>MAHHHHHHMSKINKLEQIRNIGICAHIDAGKTTTTERILYYTGKSHKIGEVHEGGATMDWMEQEQERGITITSAATTCRWQDKVINIIDTPGHVDFTIEVERSLRVLDGAVAVFDGVAGVEPQSETVWRQADKYNVPRMCFVNKMDRMGADFYRCVEMIKDRLGARSLIIQLPIGIEENFKGIVNLIKMKAVIWKDESLGAEYFEEDIPADMQDKAAEYRARLLDMVVELDDTIMEQYLSGAEITEEQIKILIRKGTIEARFYPILCGSAFKNKGVQPLLDAIVDFLPSPIDIGIVKGIEVSTSEEKDFPISIVEPFSALAFKIMNDPFVGSLTFIRIYSGKITSGATVINTVKNKREKIGRMLLMHANNREDIKEASAGDIVALAGLKDTSTGDTLSDIDKQVVLERMEFPEPVIELAVEPKSTADQEKMGLALSRLAAEDPSFRVSTDHETGQTVIKGMGELHLEIIIDRMRREFKVEANIGAPQVAYRETITTACEIDYTHKKQSGGAGQFARVKIIFEPLKDVI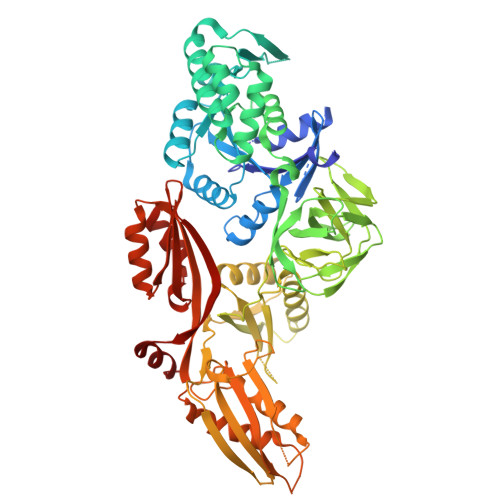DLKDEDKNKTFVFESKIVGGAVPKEYIPGVEKGLNNIRETGVIAGYPMIDFKATLVDGAFHDVDSSVLAFEIAAKGAFREGMQKGNPKLLEPIMKVEVITPDEYMGDIIGDLNSRRGQIQNMDPRGNAQVVTAHVPLAEMFGYVNTLRSLSQGRAQFSMIFSHYDQVPSQVADMIKAKK[2x]4-[[[(4~{S})-2,2-dimethyloxan-4-yl]amino]methyl]phenol 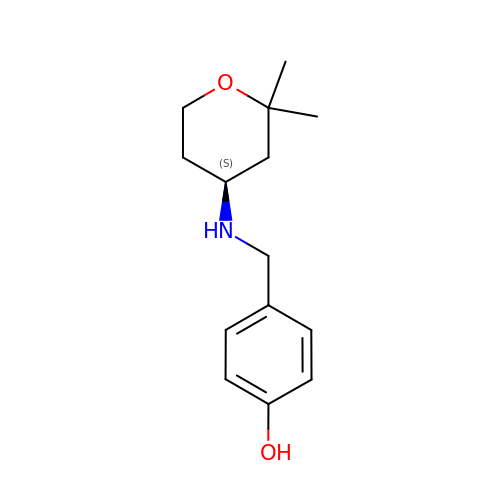| C14 H21 N O2 | PVWMKLSLRANGDD-LBPRGKRZSA-N>MAAAAAAKIAPSMLSSDFANLAAEADRMVRLGADWLHMDIMDGHFVPNLTIGAPVIQSLRK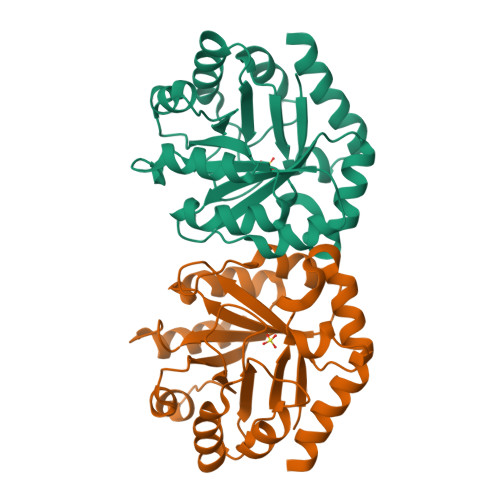HTKAYLDCHLMVTNPSDYVEPLAKAGASGFTFHIEVSRDNWQELIQSIKAKGMRPGVSLRPGTPVEEVFPLVEAENPVELVLVMTVEPGFGGQKFMPEMMEKVRALRKKYPSLDIEVDGGLGPSTIDVAASAGANCIVAGSSIFGAAEPGEVISALRKSVEGSQNKS[2x]Nonribosomal peptide synthetases (NRPSs) are multimodular enzymes that catalyze the biosynthesis of diverse peptides with a wide variety of activities. The incorporation of an acyl into peptidyl backbone is usually implemented by a starter condensation (Cs) domain, normally located at the beginning of the initial NRPS module, via the formation of an amide bond to the α-amino group of the first amino acid residue, a process also known as lipoinitiation. Genome mining of two Cs domain-embedded cryptic NRPS biosynthetic gene clusters, rzmA and holA, in the bacterium P. rhizoxinica HKI 454 resulted in the discovery of two distinct types of lipopeptides, cyclic rhizomide A (1) containing an uncommon acetyl chain (C2) and linear holrhizin A (2) harboring a medium octanoyl (C8) chain. Similar to other C domain structures reported previously, RzmA-Cs adopts a “V-shaped” configuration and consists of two subdomains (N- and C-lobes) each representing the chloramphenicol acetyltransferase (CAT) fold.

After our initial attempts to cocrystallize WT RzmA-Cs with acyl-CoAs of various lengths failed, we noticed that the R148A mutant protein showed strong binding to C8-CoA, as evidenced by the high ΔTm in protein thermal shift assays and a Kd value of ~300 nM measured using isothermal titration calorimetry (ITC). Thus we selected this mutant for crystallization, and successfully obtained both unbound and C8-CoA-bound structures. The unbound R148A structure is mostly identical to that of WT RzmA-Cs in two conformations. However, the C8-CoA-bound R148A structure shows only one conformation (in the P212121 space group), which is “tighter” than both conformations of the unbound structure, indicating that the two lobes of RzmA-Cs may close up to bind acyl-CoA substrates. The CoA portion binds at the “donor” site of Cs with its loading arm inserting into the active-site tunnel formed by two lobes, while the acyl chain turns nearly 90° and extends into the N-lobe as the R148A mutation opens up a pocket between the α5 helix (where the R148 residue is located) and the β sheet. In addition, this structure helps us understand the conservation of G145 (within the “HHxxxDG” motif), because at this position in the C domain (starting point of the α5 helix), the residue has to sacrifice its side-chain to make room for proper binding and positioning of the donor substrates. We first checked the residues near the tip of the C8 chain in the structure for mutation candidates to expand the binding pocket. Four residues, Q36 on the β1 strand, Q136 and Y138 on the β6 strand, and M143 on the loop between β6 and α5, were selected for this purpose. On the basis of the complex structure of the Cs domain with acyl-CoA and of both in vitro and in vivo mutation experiments in this investigation, we revealed the binding pocket of acyl group and the key amino acid residues that control the length of the acyl group.

> GSHMDASVMSTTYALSAAQTEIWLAQQLYPDSPVYNIAQYTVIEGVIEPAVFEAALRQVIDEADTLRLQFIDSDDGLRQRIGTPAWSMPVLDLTAQADPQAAAQAWMRADYQQPVNLTQGPLFCYALLKVAPAQWMWYQRYHHIMMDGYGAYLIAQRVAYVYSALCEGTTPAECDFGSILQLLESDAQYQISAQRAQDEAYWLKHCANWSEPATLASRSAPVLQQRLRQTTYLAIQALGDTAPDARRLAQFMTAAMAAYLYRFTGEQDVVLGLPVKVRFGADRHIPGMKSNTLPLRLTMRPGMNLSSLMQQAAQEMQSGLRHQRYPSEALRRQLGMPSGQRLFGTTVNVMPFDLDLSFGGYSATNHNLLNGPAEDLMLGVYWTPGSHQLRIDFDANPACYTPEGLGAHQRRFIRFMQVLAADATQPIDSIDLLD(5R)-N,N-DIETHYL-5-METHYL-2-[(THIOPHEN-2-YLCARBONYL)AMINO]-4,5,6,7-TETRAHYDRO-1-BENZOTHIOPHENE-3-CARBOXAMIDE 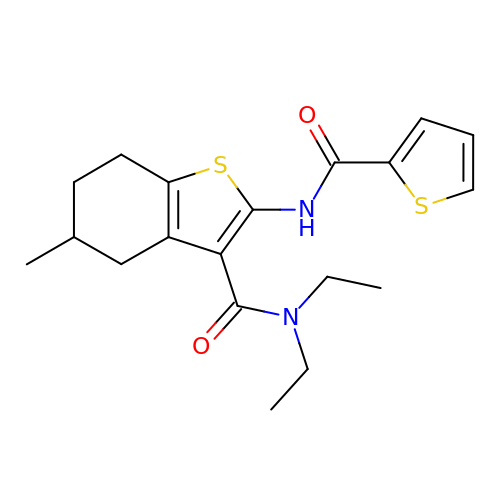| C19 H24 N2 O2 S2 | UQKSYQYWUHUIEH-GFCCVEGCSA-N> ESG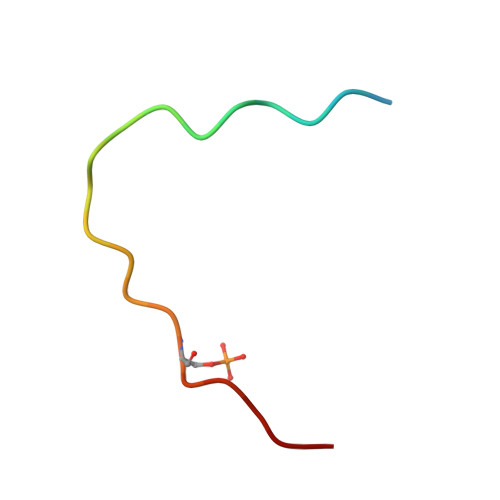LVNADLDVKDELMFSPLVDS> LMLHKRNICPIKGCGKNFFSHKYLVQHQRVHSDDRPLKCPWKGCKMTFKWAWSRTEHIRVHTGARPYVCAEPDCGQTFRFVSDFSRHKRKTGHSVKKTNKR

The RELATIVE OF EARLY FLOWERING 6 protein (REF6/JMJ12), a Jumonji C (JmjC) domain—containing histone demethylase, specifically demethylates H3K27me3 at its target loci. REF6 has intrinsic DNA-binding ability and specifically recognizes its target sequence (CTCTGYTY motif, Y = T or C) via tandem zinc-finger (ZnF) domains located at its C-terminus. ZnF domains adopt the canonical ββα fold, with a small β-sheet packed against a helix in a globular structure, and wrap more than one turn of the DNA double helix, interacting with DNA in the major groove with a classic α-helix. Structural analysis demonstrates that CHG methylation is unfavorable for REF6 binding and attenuates REF6-binding affinity.

Although the overall structures of the REF6 ZnF domains were similar between complexes with methylated or unmethylated DNA oligos, there are minor conformational changes when DNA strands carrying the methyl-group.> MPISPIETVPVKLKPGMDGPKVKQWPLTEEKIKALVEICTEMEKEGKISKIGPENPYNTPVFAIKKKDSTKWRKLVDFRELNKRTQDFWEVQLGIPHPAGLKKKKSVTVLDVGDAYFSVPLDEDFRKYTAFTIPSINNETPGIRYQYNVLPQGWKGSPAIFQSSMTKILEPFRKQNPDIVIYQYMDDLYVGSDLEIGQHRTKIEELRQHLLRWGLTTPDKKHQKEPPFLWMGYELHPDKWTVQPIVLPEKDSWTVNDIQKLVGKLNWASQIYPGIKVRQLCKLL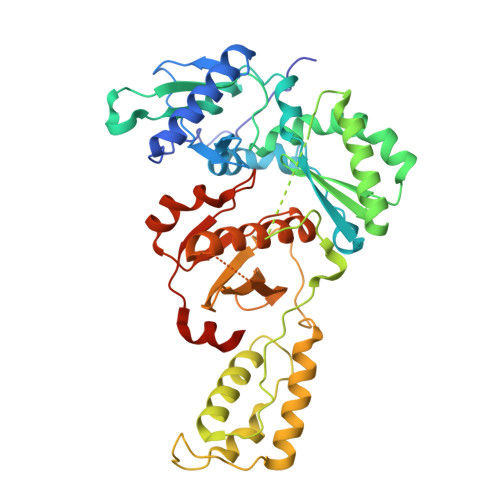RGTKALTEVIPLTEEAELELAENREILKEPVHGVYYDPSKDLIAEIQKQGQGQWTYQIYQEPFKNLKTGKYARMRGAHTNDVKQLTEAVQKITTESIVIWGKTPKFKLPIQKETWETWWTEYWQATWIPEWEFVNTPPLVKLWYQLEKEPIVGAETF7-(cyclopropylmethyl)-2-methyl-10-[(methylsulfonyl)methyl]-2,4,6,7-tetrahydro-3H-2,4,7-triazadibenzo[cd,f]azulen-3-one 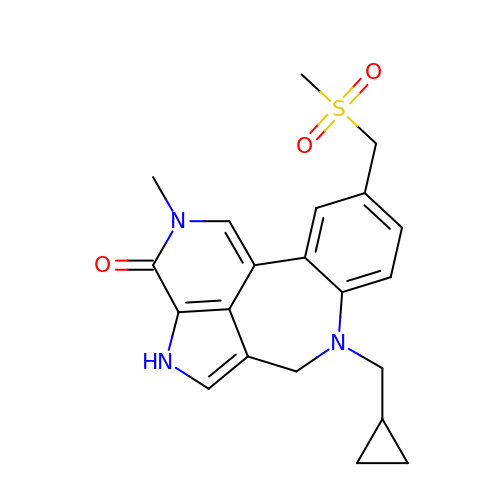| C21 H23 N3 O3 S | AGRVPCMMHQFJTH-UHFFFAOYSA-N>MECGLNNRIRMIGQICEVAKTKKFEEHAVEALWKAVADLLQPERPLEARHAVLALLKAIVQGQGERLGVLRALFFKVIKDYPSNEDLHERLEVFKALTDNGRHITYLEEELADFVLQWMDVGLSSEFLLVLVNLVKFNSCYLDEYIARMVQMICLLCVRTASSVDIEVSLQVLDAVVCYNCLPAESLPLFIVTLCRTINVKELCEPCWKLMRNLLGTHLGHSAIYNMCHLMEDRAYMEDAPLLRGAVFFVGMALWGAHRLYSLRNSPTSVLPSFYQAMACPNEVVSYEIVLSITRLIKKYRKELQVVAWDILLNIIERLLQQLQTLDSPELRTIVHDLLTTVEELCDQNEFHGSQERYFELVERCADQRPESSLLNLISYRAQSIHPAKDGWIQNLQALMERFFRSESRGAVRIKVLDVLSFVLLINRQFYEEELINSVVISQLSHIPEDKDHQVRKLATQLLVDLAEGCHTHHFNSLLDIIEKVMARSLSPPPELEERDVAAYSASLEDVKTAVLGLLVILQTKLYTLPASHATRVYEMLVSHIQLHYKHSYTLPIASSIRLQAFDFLLLLRADSLHRLGLPNKDGVVRFSPYCVCDYMEPERGSEKKTSGPLSPPTGPPGPAPAGPAVRLGSVPYSLLFRVLLQCLKQESDWKVLKLVLGRLPESLRYKVLIFTSPCSVDQLCSALCSMLSGPKTLERLRGAPEGFSRTDLHLAVVPVLTALISYHNYLDKTKQREMVYCLEQGLIHRCASQCVVALSICSVEMPDIIIKALPVLVVKLTHISATASMAVPLLEFLSTLARLPHLYRNFAAEQYASVFAISLPYTNPSKFNQYIVCLAHHVIAMWFIRCRLPFRKDFVPFITKGLRSNVLLSFDDTPEKDSFRARSTSLNERPKSRIQTSLTSASLGSADENSVAQADDSLKNLHLELTETCLDMMARYVFSNFTAVPKRSPVGEFLLAGGRTKTWLVGNKLVTVTTSVGTGTRSLLGLDSGELQSGPESSSSPGVHVRQTKEAPAKLESQAGQQVSRGARDRVRSMSGGHGLRVGALDVPASQFLGSATSPGPRTAPAAKPEKASAGTRVPVQEKTNLAAYVPLLTQGWAEILVRRPTGNTSWLMSLENPLSPFSSDINNMPLQELSNALMAAERFKEHRDTALYKSLSVPAASTAKPPPLPRSNTDSAVVMEEGSPGEVPVLVEPPGLEDVEAALGMDRRTDAYSRSSSVSSQEEKSLHAEELVGRGIPIERVVSSEGGRPSVDLSFQPSQPLSKSSSSPELQTLQDILGDPGDKADVGRLSPEVKARSQSGTLDGESAAWSASGEDSRGQPEGPLPSSSPRSPSGLRPRGYTISDSAPSRRGKRVERDALKSRATASNAEKVPGINPSFVFLQLYHSPFFGDESNKPILLPNESQSFERSVQLLDQIPSYDTHKIAVLYVGEGQSNSELAILSNEHGSYRYTEFLTGLGRLIELKDCQPDKVYLGGLDVCGEDGQFTYCWHDDIMQAVFHIATLMPTKDVDKHRCDKKRHLGNDFVSIVYNDSGEDFKLGTIKGQFNFVHVIVTPLDYECNLVSLQCRKDMEGLVDTSVAKIVSDRNLPFVARQMALHANMASQVHHSRSNPTDIYPSKWIARLRHIKRLRQRICEEAAYSNPSLPLVHPPSHSKAPAQTPAEPTPGYEVGQRKRLISSVEDFTEFV[2x];>[2x]MAQQANVGELLAMLDSPMLGVRDDVTAVFKENLNSDRGPMLVNTLVDYYLETSSQPALHILTTLQEPHDKHLLDRINEYVGKAATRLSILSLLGHVIRLQPSWKHKLSQAPLLPSLLKCLKMDTDVVVLTTGVLVLITMLPMIPQSGKQHLLDFFDIFGRLSSWCLKKPGHVAEVYLVHLHASVYALFHRLYGMYPCNFVSFLRSHYSMKENLETFEEVVKPMMEHVRIHPELVTGSKDHELDPRRWKRLETHDVVIECAKISLDPTEASYEDGYSVSHQISARFPHRSADVTTSPYADTQNSYGCATSTPYSTSRLMLLNMPGQLPQTLSSPSTRLITEPPQATLWSPSMVCGMTTPPTSPGNVPPDLSHPYSKVFGTTAGGKGTPLGTPATSPPPAPLCHSDDYVHISLPQATVTPPRKEERMDSARPCLHR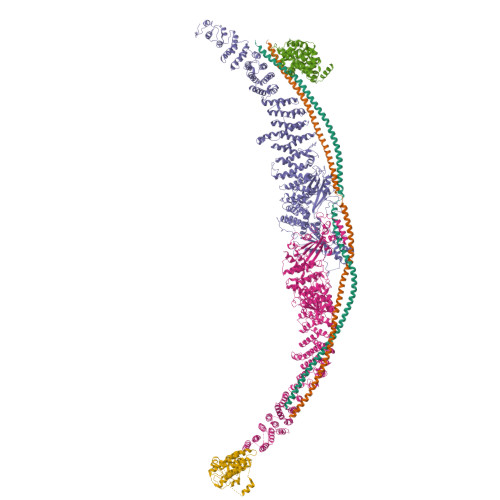QHHLLNDRGSEEPPGSKGSVTLSDLPGFLGDLASEEDSIEKDKEEAAISRELSEITTAEAEPVVPRGGFDSPFYRDSLPGSQRKTHSAASSSQGASVNPEPLHSSLDKLGPDTPKQAFTPIDLPCGSADESPAGDRECQTSLETSIFTPSPCKIPPPTRVGFGSGQPPPYDHLFEVALPKTAHHFVIRKTEELLKKAKGNTEEDGVPSTSPMEVLDRLIQQGADAHSKELNKLPLPSKSVDWTHFGGSPPSDEIRTLRDQLLLLHNQLLYERFKRQQHALRNRRLLRKVIKAAALEEHNAAMKDQLKLQEKDIQMWKVSLQKEQARYNQLQEQRDTMVTKLHSQIRQLQHDREEFYNQSQELQTKLEDCRNMIAELRIELKKANNKVCHTELLLSQVSQKLSNSESVQQQMEFLNRQLLVLGEVNELYLEQLQNKHSDTTKEVEMMKAAYRKELEKNRSHVLQQTQRLDTSQKRILELESHLAKKDHLLLEQKKYLEDVKLQARGQLQAAESRYEAQKRITQVFELEILDLYGRLEKDGLLKKLEEEKAEAAEAAEERLDCCNDGCSDSMVGHNEEASGHNGETKTPRPSSARGSSGSRGGGGSSSSSSELSTPEKPPHQRAGPFSSRWETTMGEASASIPTTVGSLPSSKSFLGMKARELFRNKSESQCDEDGMTSSLSESLKTELGKDLGVEAKIPLNLDGPHPSPPTPDSVGQLHIMDYNETHHEHS;> GVEEKKSLEILLKDDRLDTEKLCTFSQRFPLPSMYRALVWKVLLGILPPHHESHAKVMMYRKEQYLDVLHALKVVRFVSDATPQAEVYLRMYQLESGKLPRSPSFPLEPDDEVFLAIAKAMEEMVEDSVDCYWITRRFVNQLNTKYRDSLPQLPKAFEQYLNLEDGRLLTHLRMCSAAPKLPYDLWFKRCFAGCLPESSLQRVWDKVVSGSCKILVFVAVEILLTFKIKVMALNSAEKITKFLENIPQDSSDAIVSKAIDLWHKHCG>MDYNVKDFGALGDGVSDDRASIQAAIDAAYAAGGGTVYLPAGEYRVSAAGEPGDGCLMLKDGVYLAGAGMGETVIKLIDGSDQKITGMVRSAYGEETSNFGMRDLTLDGNRDNTSGKVDGWFNGYIPGGDGADRDVTIERVEVREMSGYGFDPHEQTINLTIRDSVAHDNGLDGFVADYLVDSVFENNVAYANDRHGFNVVTSTHDFVMTNNVAYGNGSSGLVVQRGLEDLALPSNILIDGGAYYDNAREGVLLKMTSDITLQNADIHGNGSSGVRVYGAQDVQILDNQIHDNAQ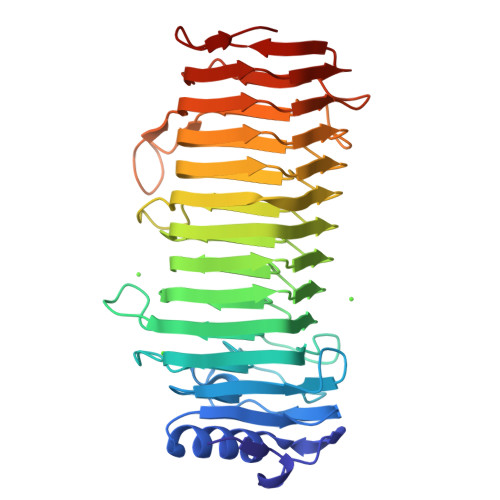AAAVPEVLLQSFDDTAGASGTYYTTLNTRIEGNTISGSANSTYGIQERNDGTDYSSLIDNDIAGVQQPIQLYGPHSTVSGEP[2x]> GSHMASMTGGQQMGRGSE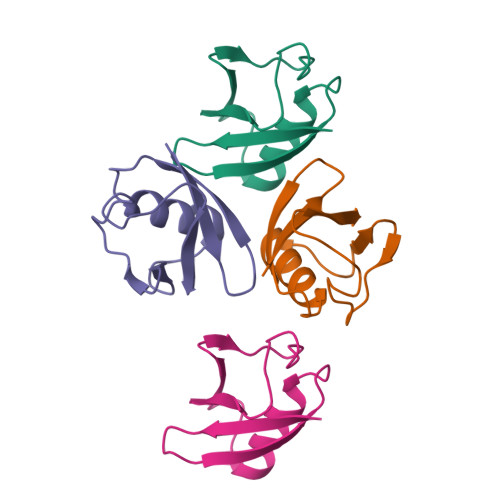FTENNDHINLKVAGQDGSVVQFKIKRHTPLSKLMKAYCERQGLSMRQIRFRFDGQPINETDTPAQLEMEDEDTIDVFQQQTGGL> SVDFKTYVDQACRAAEEFVNVYYTTMDK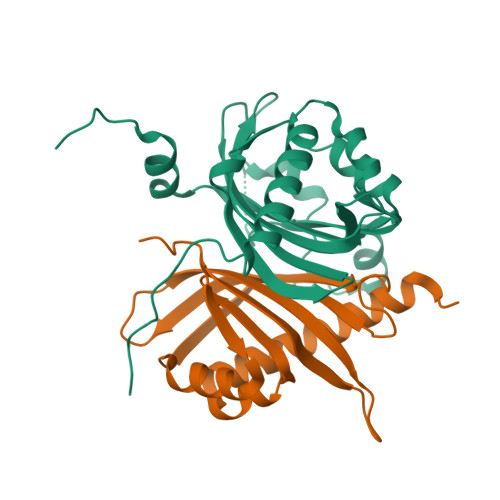RRRLLSRLYMGTATLVWNGNAVSGQESLSEFFEMLPSSEFQISVVDCQPVHDEATPSQTTVLVVICGSVKFEGNKQRDFNQNFILTAQASPSNTVWKIASDCFRFQDWAS;> APTTLPPCKGSYFGTENLKSLVLHFLQQYYAIYDSGDRQGLLDAYHDGACCSLSIPFIPQNPARSSLAEYFKDSRNVKKLKDPTLRFRLLKHTRLNVVAFLNELPKTQHDVNSFVVDISAQTSTLLCFSVNGVFKEVDGKSRDSLRAFTRTFIAVPASNSGLCIVNDELFVRNASSEEIQRAFAMPAPTP>AELCNKQQQQGPFTFANYQESPLNVSRLQIKVTKTTVQDRGKNFIIGYRAYWRSYCYNGGSLDGNTGCYNSLNPKPPTKDELKTWGQEEVCYTGPEVQDAWSGDSSICFVDWKMDNKHRAKELEKRSNNNHFAHHTCNLSWRCGVTNTHLEVRLVASGTQPQAVIVMPNGTTRAVSMVAETFWTDGEFSYLYSPKVFGTRAETKFIPCFKEHVKTRLDQGGSDYLIHDLTTEKFHCKDGDNFFEFPSSGFICLPDACYKNEKQKNNLLHPGMWNISEKLHAASVYDVNNVIHSLVYETESLRLSLAQLDHRFSVLTKLMNKMVSSLAKIDDRLIGALLEKPMASKFISPTKFMVSPCVAVLEEESNC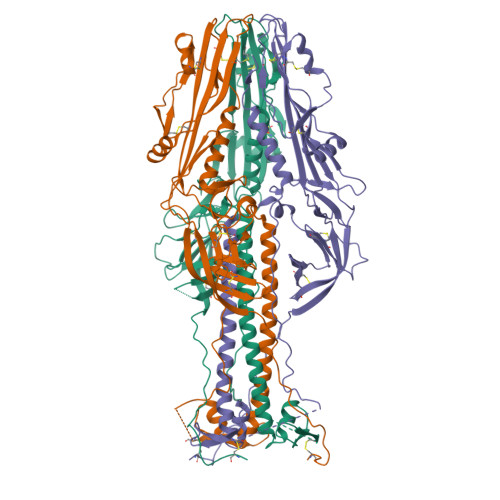HKDSIYRDGRWVYNNDPTKCFILNSSQTIDLFNFKTLWLPQLVAAKVEGVVSDEDGWTFVANSKQALLDTMTYTKNGGRGTSMEDVLNYPSGWLSGKLNG[3x]>LAFPKEFWWGGATSGPQSEGRFAKQHRNLFDYWYEEEPDLFYDYVGPDTASDAYHQIESDLTLLASLGHNSYRTSIQWTRLIDDFEQATINPDGLAYYNRVIDACLANGIRPVINLHHFDLPIALYQAYGGWESKHVVDLFVAFSKVCFEQFGDRVKDWFVHNEPMVVVEGSYLMQFHYPAIVDGKKAVQVAYNLALATAKVIQAYRRGPAELSDGRIGTILNLTPAYPASQSEADMAAAHFAELWNNDLFMEAAVHGKFPEELVAVLKKDGVLWQSTPEELALIAENRVDYLGLNFYHPKRVKAPDAIPVISPSWSPEWYYDPYLMPGRRMNVDKGWEIYPEAVYDIAIKMRDHYDNIPWFLSENGVGISGEDRYRDETGQIQDDYRIQFLKEHLTYLHKGIEAGSNCFGYHVWTPIDGWSWLNAYKNRYGLVENNIHTQVRRPKASAYWFKKVATHNRLISLEVME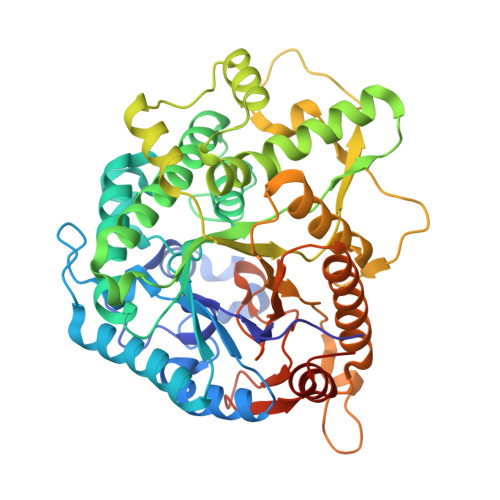EFGGSASHLSD[6x]> ATIFG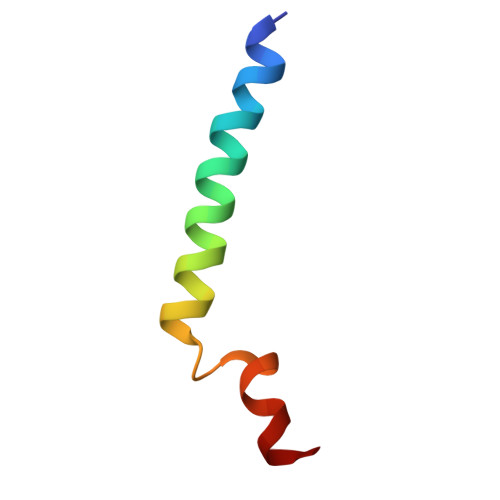GAFAFQGFFDVAVNKWWEEHNKAKLWKNVKGKFL>[2x]SMHSDLTFCEIILMEMESHDAAWPFLEPVNPRLVSGYRRIIK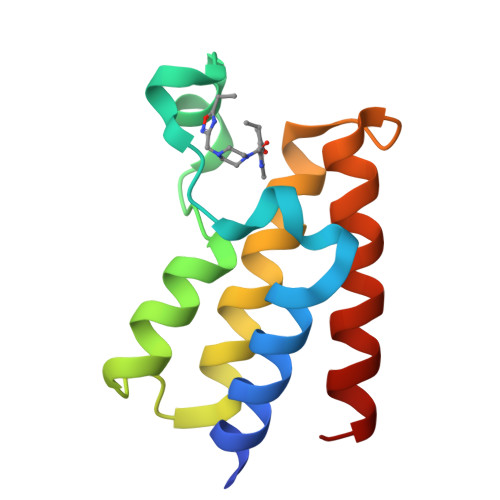NPMDFSTMRERLSRGGYTSSEEFAADALLVFDNCQTFNEDDSEVGKAGHIMRRFFESRWEEFY> CDIPQSTNCGGNVYSNDDINTAIQGALDDVANGDRPDNYPHQYY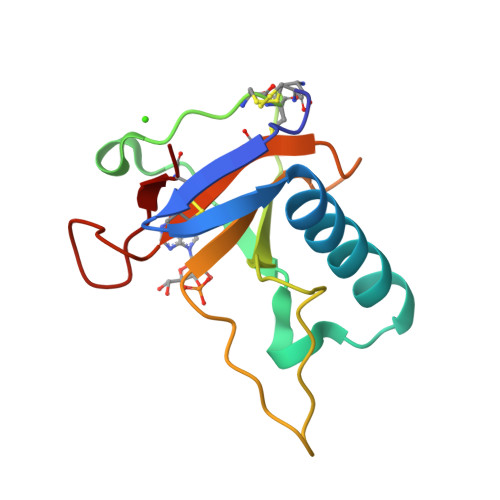DEASEDITLCCGSGPWSEFPLVYNGPYYSSRDNYVSPGPDRVIYQTNTGEFCATVTHTGAASYDGFTQCS> LTAKHRPSVVWLHNAECTGCTEAAIRTIKPYIDALILDTISLDYQETIMAAAGEAAEAALHQALEGKDGYYLVVEGGLPTIDGGQWGMVAGHPMIETTKKAAAKAKGIICIGTCSAYGGVQKAKPNPSQAKGVSEALGVKTINIPGCPPNPINFVGAVVHVLTKGIPDLDENGRPKLFYGELVHDNCPRLPHFEASEFAPSFDSEEAKKGFCLYELGCKGPVTYNNCPKVLFNQVN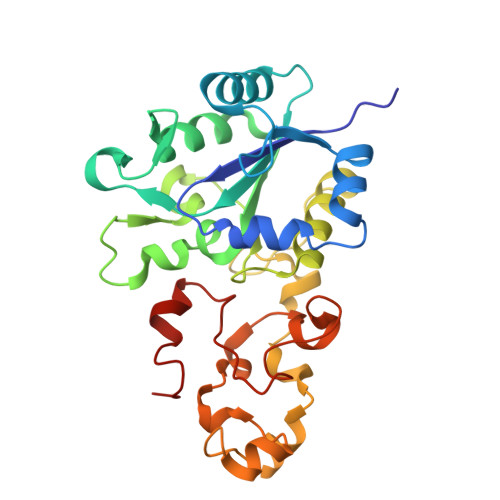WPVQAGHPCLGCSEPDFWDTMTPFYEQG>[2x]MSEQSYRSAGTLLAQLASGETTSVALVNHYFSRMAQFNKPLNAVVQQHYALALEAAARADRERLEGRARGVLHGLPCTVKESFDVQGWLTTSGAHYLKDNRATQDAPS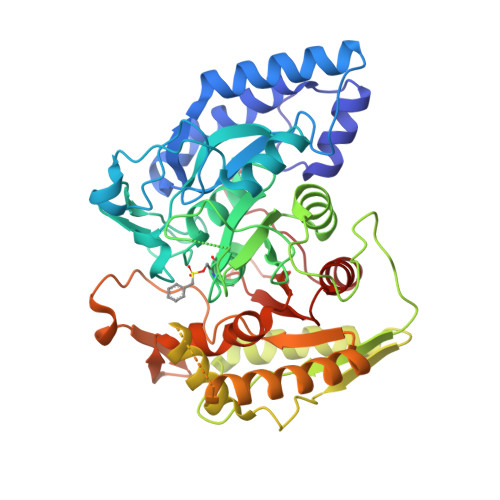IARLRAAGAILMGKTNVPMMTADWQTYNDLYGTTHNLWDRQRSPGGSSGGAAVAVAADFTPVEFGSDLFGSLRIPAHYTGVYAHRCSLGLMSVRGHVPGGGPQATDEPDLSTAGPMARSAADLRLMMRALSTFWVEPPRIPDFSRYQAKANYRVCTWFSAPHHEIDQQIAQRFQSFIDKLRAQPGVEVDDAMPADIDPDALFDIAVKLSGRLVSTALNGRQRLTAGLAALGFRLVGKLADVPEGITSYYQGMLKDSGEQRNTDKLRHEYSRVIETLFARYDVLLTPVSPVLAFAHMQQPVRKRKLIVNGEPQDYNEHLFWNMLATVFGLPATVYPLAKTMDELPCGIQIISGHFHDDVTINFAEFCESISGGFTVPEGYG> MQNAESWFKKYWHLSVLVIAALISVKLRILNPWNSVFTWTVRLGGNDPWYYYRL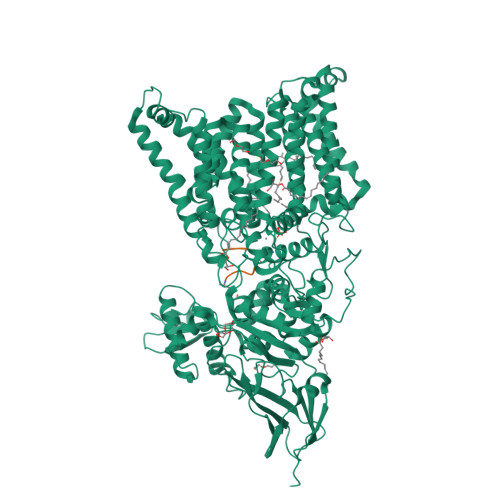IENTIHNFPHRIWFDPFTYYPYGSYTHFGPFLVYLGSIAGIIFSATSGESLRAVLAFIPAIGGVLAILPVYLLTREVFDKRAAVIAAFLIAIVPGQFLQRSILGFNDHHIWEAFWQVSALGTFLLAYNRWKGHDLSHNLTARQMAYPVIAGITIGLYVLSWGAGFIIAPIILAFMFFAFVLAGFVNADRKNLSLVAVVTFAVSALIYLPFAFNYPGFSTIFYSPFQLLVLLGSAVIAAAFYQIEKWNDVGFFERVGLGRKGMPLAVIVLTALIMGLFFVISPDFARNLLSVVRVVQPKGGALTIAEVYPFFFTHNGEFTLTNAVLHFGALFFFGMAGILYSAYRFLKRRSFPEMALLIWAIAMFIALWGQNRFAYYFAAVSAVYSALALSVVFDKLHLYRALENAIGARNKLSYFRVAFALLIALAAIYPTYILADAQSSYAGGPNKQWYDALTWMRENTPDGEKYDEYYLQLYPTPQSNKEPFSYPFETYGVISWWDYGHWIEAVAHRMPIANPFQAGIGNKYNNVPGASSFFTAENESYAEFVAEKLNVKYVVSDIEMETCKYYAMAVWAEGDLPLAEKYYGGYFYYSPTGTFGYANSQWDIPLNSIIIPLRIPSELYYSTMEAKLHLFDGSGLSHYRMIYESDYPAEWKSYSSQVNLNNESQVLQTALYEAVMRARYGVSPTMGTQEVLYKYAYTQLYEKKMGIPVKIAPSGYVKIFERVKGAVVTGKVSANVTEVSVNATIKTNQNRTFEYWQTVEVKNGTYTVVLPYSHNSDYPVKPITPYHIKAGNVVKEITIYESQVQNGEIIQLDLELALVPR;> APYAVTASCR5’-Cytosolic nucleotidase IIIB (cN-IIIB) is one of the most recently discovered 5’-nucleotidases and has several unique structural and functional features. However, one of the most preferred cN-IIIB substrates is m7GMP, for which the activity of dephosphorylation is characterized by one order of magnitude lower KM constant compared to the other preferred substrates, whereas kcat/KM is comparable. The crystal structure of cN-IIIB consists of two distinct domains: the globular core domain (residues 1–51, 132–182, and 215–300) and the smaller CAP domain (52–131 and 183–214). The core domain is a haloacid dehalogenase domain (HAD).

In the structure of cN-IIIB in complex with 3,4-diF-Bn7GMP (5d), each moiety of the inhibitor is stabilized by direct contact with various protein residues. The 3,4-difluorobenzyl group of the modified base is accommodated in a hydrophobic cavity formed by sidechains of Trp105, Trp106, Tyr 60, Ala109, Leu63, Leu77, Leu113, and Ile159. Then, the guanine base intercalates between the off-centered π-ring system of Tyr 60 and Trp105 separated by typical stacking distances of 3.6 Å between the side chains and the base. The hydroxyl group of Tyr 60 is additionally engaged in interacting with the ribose ring, which adopts O-4’-endo conformation. Tyr 60 forms a hydrogen bond with the O4’ atom, while the 2’- and 3’-oxygens of the ribose are hydrogen bonded with the carboxylic group of highly conserved Glu 88. The phosphate group is placed in a binding cavity in the vicinity of amine group of Lys205 and amide group of Ala157, which are in direct contact with phosphate oxygens. Additional hydrogen bonds via structural water molecule with hydroxyl residue of Ser156 and hydrogen bond of Tyr60 with 5’-O-oxygen support the stabilizing contact of phosphate group with nucleotidase and simultaneously distance it from the catalytic center by 2.7 Å. The observed shift of the phosphate center away from the catalytic site may explain why the compound does not undergo dephosphorylation despite tight binding to the protein. The differences between solved structures: the holoenzyme of cN-IIIB • Mg2+, and the enzyme in complex with inhibitors: 5d or 5d’, concern mainly two helices of the CAP domain, which move slightly down and left towards HAD domain by about 3 Å. Comparisons CAP of domains revealed that human cN-IIIB stays in a more open conformation than the domain of Drosophila cN-IIIB. All the above suggest that ligand 5d freezes the protein conformation in an open state of the enzyme.

>RSMAEEVSTLMKATVLMRQPGRVQEIVGALRKGGGDRLQVISDFDMTLSRFAYNGKRCPSSYNILDNSKIISEECRKELTALLHHYYPIEIDPHRTVKEKLPHMVEWWTKAHNLLCQQKIQKFQIAQVVRESNAMLREGYKTFFNTLYHNNIPLFIFSAGIGDILEEIIRQMKVFHPNIHIVSNYMDFNEDGFLQGFKGQLIHTYNKNSSACENSGYFQQLEGKTNVILLGDSIGDLTMADGVPGVQNILKIGFLNDKVEERRERYMDSYDIVLEKDETLDVVNGLLQHILCQGVQLEMQGP[2x]>FVVRDIRVNGLVRLTPANVYTMLPINSGDRVNEPMIAEAIRTLYATGLFDDIKASKENDTLVFNVIERPIISKLEFKGNKLIPKEALEQGLKKMGIAEGEVFKKSALQTIETELEQQYTQQGRYDADVTVDTVARPNNRVELKINFNEGTPAKVFDINVIGNTVFKDSEIKQAFAVKESGWASVVTRNDRYAREKMAASLEALRAMYLNKGYINFNINNSQLNISEDKKHIFIEV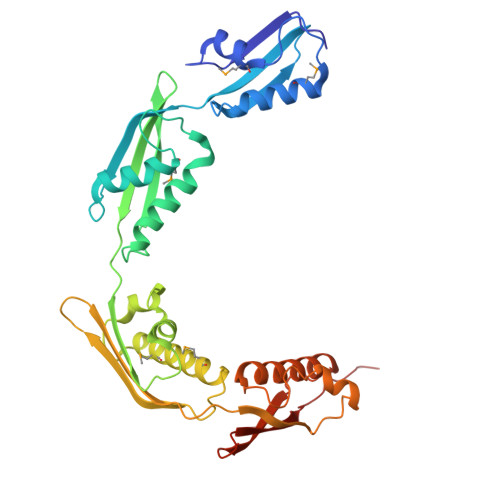AVDEGSQFKFGQTKFLGDALYKPEELQALKIYKDGDTYSQEKVNAVKQLLLRKYGNAGYYFADVNIVPQINNETGVVDLNYYVNPGQQVTVRRIN[2x]> SMRICIFMARGLEGCGVTKFSLEQR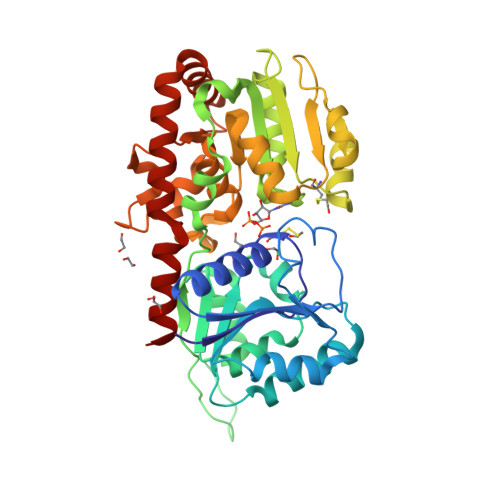DWFIKNGHEVTLVYAKDKSFTRTSSHDHKSFSIPVILAKEYDKALKLVNDCDILIINSVPATSVQEATINNYKKLLDNIKPSIRVVVYQHDHSVLSLRRNLGLEETVRRADVIFSHSDNGDFNKVLMKEWYPETVSLFDDIEEAPTVYNFQPPMDIVKVRSTYWKDVSEINMNINRWIGRTTTWKGFYQMFDFHEKFLKPAGKSTVMEGLERSPAFIAIKEKGIPYEYYGNREIDKMNLAPNQPAQILDCYINSEMLERMSKSGFGYQLSKLNQKYLQRSLEYTHLELGACGTIPVFWKSTGENLKFRVDNTPLTSHDSGIIWFDENDMESTFERIKELSSDRALYDREREKAYEFLYQHQDSSFCFKEQFDIITK> GGGGRSVDTMALWLGLRAVLVVAGLAVLLQLIRGWLSSKSYVFNREEIARLAKEHSGLDYEVAFSKIIVELRKKHPGHILQDEDLQWVFVNAGGWMGSMCLLHASLTEYVLLFGTAVDTGGHSGRYWAEISDTILSGTFRQWKEGTTKSEIFYPGDTIVHEVGEATSVQWSSGTWMVEYGRGFIPSTLAFALADTIFSTQDFLTLFYTVKVYSKALLLEASTHLSQLGFFAAA

The sigma-1 receptor (σ1R) is an endoplasmic reticulum (ER)-localized, non-opioid transmembrane receptor implicated in many pathological conditions, including neurodegenerative disorders and cancer. So far, all reported σ1R structures are homotrimers, with the ligand binding site located inside the β-barrel domain of each σ1R monomer. The ligand binding site is located in the lumen of the β-barrel domain (β1-β10), whose opening is covered by two membrane-adjacent helices (α4/α5) at the carboxy-terminus. Here, we present crystal structures of σ1R from Xenopus laevis (xlσ1R) bound to two endogenous neurosteroid ligands, progesterone (a putative antagonist) and dehydroepiandrosterone sulfate (DHEAS) (a putative agonist), at 2.15-3.09  Å resolutions.

Fortunately, co-crystallization of the xlσ1R-progesterone complex produced higher-quality crystals that diffracted to ~2 Å and its structure was solved to 2.15 Å (termed xlσ1Rprog-co). The xlσ1Rprog-co structure was solved in the I432 space group with one xlσ1R protomer per asymmetric unit, and three xlσ1R protomers form a homotrimer. However, distinct from the tadpole-shaped density in xlσ1Runknown-lig, the electron density in the ligand binding site of xlσ1Rprog-co resembles a fish with a small head, a wide body and a short tail. Meanwhile, the 2.15 Å-resolution structure of xlσ1Rprog-co readily allowed a clear placement of a progesterone molecule into the fish-shaped density. The C3 carbonyl oxygen on A-ring of progesterone occupies the fish-shape’s head proximal to the ER membrane, whereas the C17 keto methyl group on D-ring occupies the fish-shape’s tail reaching towards the distal space of the β-barrel lumen. Progesterone binds slightly closer towards the membrane, mainly through hydrophobic interactions with W86 (β2), M90 (β2), L92 (β2), Y100 (β3), L102 (β3), F104 (β3), Y117 (β4/β5 loop), I175 (α4), F181 (α4), A182 (α4), and Y203 (α5). Interestingly, electron densities corresponding to six water molecules (Water403, 404, 434, 447, 473, and 474) were observed within the distal space of the β-barrel lumen. In xlσ1Rprog-co, these water molecules form extensive hydrogen bonds with each other and with the hydrophilic patches in the distal region of the β-barrel lumen, including S114 (β4/β5 loop), Y117 (β4/β5 loop), D123 (β5), Q132 (β6), H151 (β8), and T157 (β9). Water403 also forms a direct hydrogen bond with the C20 carbonyl oxygen of the progesterone tail. Thus, this water-mediated hydrogen bond network connects bound progesterone indirectly to the receptor.>[4x]SRPLSDQEKRKQISVRGLAGVENVTELKKNFNRHLHFTLVKDRNVATPRDYYFALAHTVRDHLVGRWIRTQQHYYEKDPKRIYYLSLEFYMGRTLQNTMVNLALENACDEATYQLGLDMEELEEIEEDAGLGNGGLGRLAACFLDSMATLGLAAYGYGIRYEFGIFNQKICGGWQMEE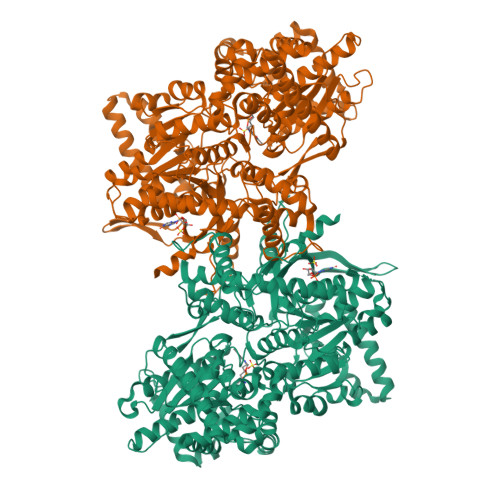ADDWLRYGNPWEKARPEFTLPVHFYGRVEHTSQGAKWVDTQVVLAMPYDTPVPGYRNNVVNTMRLWSAKAPNDFNLKDFNVGGYIQAVLDRNLAENISRVLYPNDNFFEGKELRLKQEYFVVAATLQDIIRRFKSSKFGCRDPVRTNFDAFPDKVAIQLNDTHPSLAIPELMRVLVDLERLDWDKAWEVTVKTCAYTNHTVIPEALERWPVHLLETLLPRHLQIIYEINQRFLNRVAAAFPGDVDRLRRMSLVEEGAVKRINMAHLCIAGSHAVNGVARIHSEILKKTIFKDFYELEPHKFQNKTNGITPRRWLVLCNPGLAEIIAERIGEEYISDLDQLRKLLSYVDDEAFIRDVAKVKQENKLKFAAYLEREYKVHINPNSLFDVQVKRIHEYKRQLLNCLHVITLYNRIKKEPNKFVVPRTVMIGGKAAPGYHMAKMIIKLITAIGDVVNHDPVVGDRLRVIFLENYRVSLAEKVIPAADLSEQISTAGTEASGTGNMKFMLNGALTIGTMDGANVEMAEEAGEENFFIFGMRVEDVDRLDQRGYNAQEYYDRIPELRQIIEQLSSGFFSPKQPDLFKDIVNMLMHHDRFKVFADYEEYVKCQERVSALYKNPREWTRMVIRNIATSGKFSSDRTIAQYAREIWGVEPSRQRLPAPDEKIP> MAETDGSIPLIPVRMLNEHVYCPRLAYLMWVQGEFSHNEFTVDGVIRHRRVDAGGGVLPSETQEDSRIHARSVSLSSERLGITAKIDLVEGEGAYVSPVDYKRGKRPHVAGGAYEPERVQLCAQGLLLREHGFASDGGALYFVASRERVPVAFDDELIGRTLAAIDEMGRTALSGTMPPPLEDSPKCPRCSLVGICLPDEVRFLSHLSVEPRPIIPADGRGLPLYVQSPKAYVR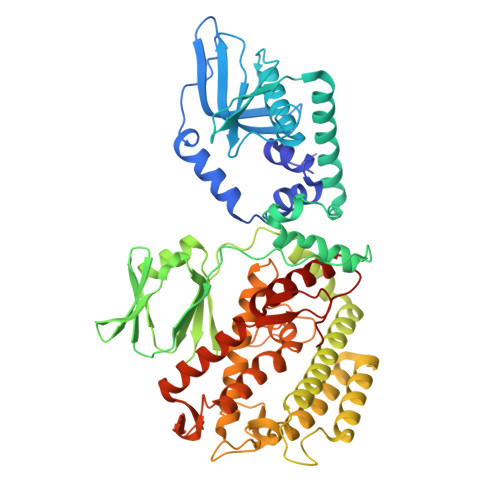KDGDCLVIEEERVRVAEARLGETSQVALFGNATLTTAALHECLRREIPVTWLSYGGWFMGHTVSTGHRNVETRTYQYQRSFDPETCLNLARRWIVAKIANCRTLLRRNWRGEGDEAKAPPGLLMSLQDDMRHAMRAPSLEVLLGIEGASAGRYFQHFSRMLRGGDGEGMGFDFTTRNRRPPKDPVNALLSFAYAMLTREWTVALAAVGLDPYRGFYHQPRFGRPALALDMMEPFRPLIADSTVLMAINNGEIRTGDFVRSAGGCNLTDSARKRFIAGFERRMEQEVTHPIFKYTISYRRLLEVQARLLTRYLSGEIPAYPNFVTR> DHLDDSWVTVFGFPQASASYIL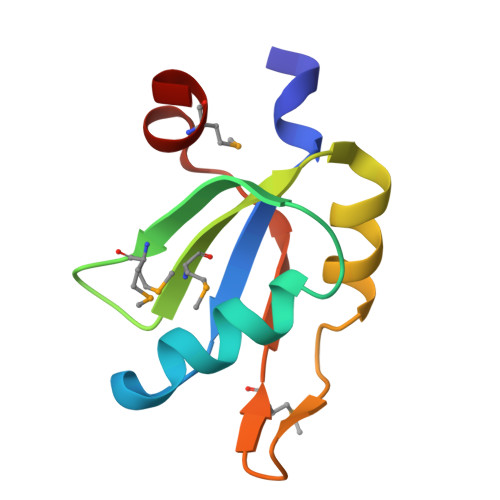LQFAQYGNILKHVMSNTGNWMHIRYQSKLQARKALSKDGRIFGESIMIGVKPCIDKSVMESS> GPLGSMSDENKSTPIVKASDITDKLKEDILTISKDALDKYQLERDIAGTVKKQLDVKYGNTWHVIVGKNFGSYVTHEKGHFVYFYIGPLAFLVFKT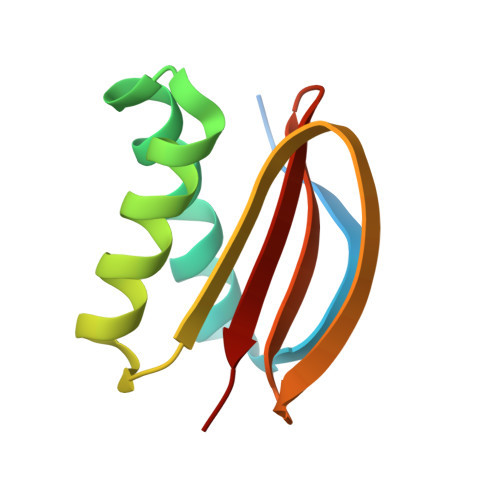A>MKTIIINGVQFNTDEDTTILKFARDNNIDISALCFLNNCNNDINKCEICTVEVEGTGLVTACDTLIEDGMIINTNSDAVNEKIKSRISQLLDIHEFKCGPCNRRENCEFLKLVIKYKARASKPFLPKDKTEYVDERSKSLTVDRTKCLLCGRCVNACGKNTETYAMKFLNKNGKTIIGAEDEKCFDDTNCLLCGQCIIACPVAALSEKSHMDRVKNALNAPEKHVIVAMAPSVRASIGELFNMGFGVDVTGKIYTALRQLGFDKIFDINFGADMTIMEEATELVQRIENNGPFPMFTSDCPGWVRQAENYYPELLNNLSSAKSPQQIFGTASKTYYPSISGLDPKNVFTVTVMPCTSKKFEADRPQMEKDGLRDIDAVITTRELAKMIKDAKIPFAKLEDSEADPAMGEYSGAGAIFGATGGVMEAALRSAKDFAENAELEDIEYKQVRGLNGIKEAEVEINNNKYNVAVINGASNLFKFMKSGMINEKQYHFIEVMACHGGCVNGGGQPHVNPKDLEKVDIKKVRASVLYNQDEHLSKRKSHENTALVKMYQNYFGKPG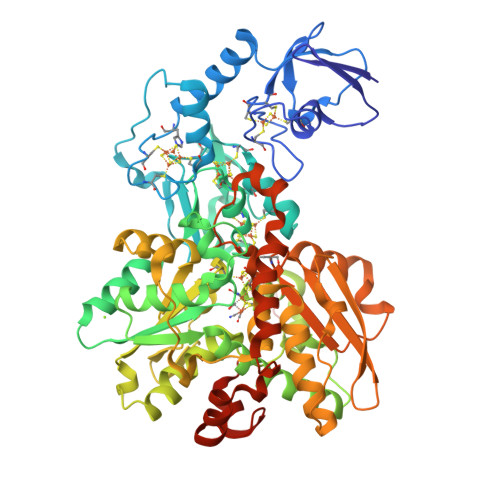EGRAHEILHFKYKKSAWSHPQFEK[2x]>[4x]SANMTHLLETFEMSIDHQEDGLVVISMPVTDKVKAPFGYLHGGASIALGETACSLGSANLIDTTKFIPLGLEMNA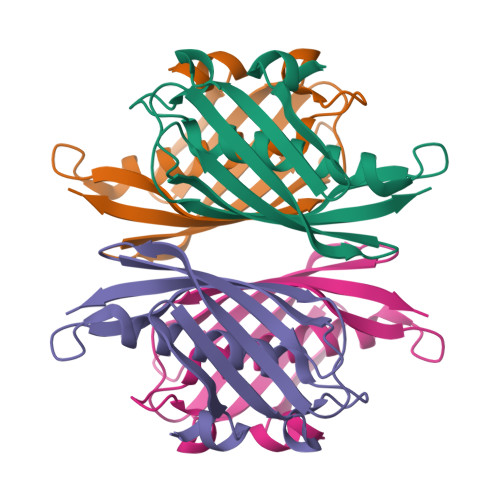NHIHSAKDGRVTATAEIIHRGKSTHVWDIKIKNDKEQLITVMRGTVAIKPLK> MGVYDYKNFGTADSKALFSDAMAITLYSYHNLDNGFAAGYQHNGFGLGLPATLVTALLGGTDSQGVIPGIPWNPDSEKLALDAVKKAGWTPITASQLGYDGKTDARGTFFGEKAGYTTAQVEILGKYDAQGHLTEIGIAFRGTSGPRENLILDSIGDVINDLLAAFGPKDYAKNYVGEAFGNLLNDVVAFAKANGLSGKDVLVSGHSLGGLAVNSMADLSGGKWGGF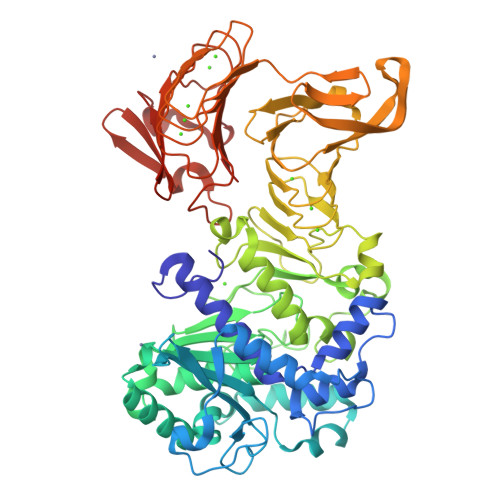FADSNYIAYASPTQSSTDKVLNVGYENDPVFRALDGSTFTGASVGVHDAPKESATDNIVSFNDHYASTAWNLLPFSILNIPTWISHLPTAYGDGMNRIIESKFYDLTSKDSTIIVANLSDPARANTWVQDLNRNAETHKGSTFIIGSDSNDLIQGGSGNDYLEGRAGNDTFRDGGGYNVILGGAGNNTLDLQKSVNTFDFANDGAGNLYVRDANGGISITRDIGSIVTKEPGFLWGLFKDDVTHSVTASGLKVGSNVTQYDASVKGTNGADTLKAHAGGDWLFGLDGNDHLIGGVGNDVFVGGAGNDLMESGGGADTFLFNGAFGQDRVVGFTSNDKLVFLGVQGVLPNDDFRAHASMVGQDTVLKFGGDSVTLVGVALNSLSADGIVIA We have recently identified interactions between two groups of Drosophila IgSF (immunoglobulin superfamily) cell adhesion molecules with properties closely matching a neuronal chemoaffinity function: 21 Dpr proteins, named after the founding member Defective proboscis extension response, selectively bind nine proteins, now called the Dpr-interacting proteins, or DIPs. All 21 Dprs and nine DIPs are predicted to contain two and three immunoglobulin (IG) domains, respectively. Our previous work identified the first IG domains, termed IG1, as the domains mediating the Dpr–DIP interaction by the formation of a pseudo-symmetric IG1-IG1 heterocomplex using the GFCC’C’ face of the immunoglobulin fold. Therefore, Dprs and DIPs are strong candidates for a synapse specification or targeting function.

We determined the crystal structure of Dpr10 IG1 bound to DIP-α IG1 and compared it to our Dpr6–DIP-α structure. The IG1 of Dpr6 and Dpr10 are 75% identical in sequence, and the interface only has three residues out of 19 that are different between Dpr6 and Dpr10. The two complex structures closely match each other, and unlike the differences among complexes described above, rotamers are nearly all conserved at the two interfaces. The differences in sequence are accommodated by small movements in surrounding side chains and do not propagate further. Overall, these results suggest that Dprs that are highly similar in sequence (≥70% identity) are unlikely to be differentiated in their DIP binding, but in time and place of expression. The high-resolution Dpr10–DIP-α structure also allowed us to observe an ordered, near-complete N-linked glycan at the interface. As we use lepidopteran cells to express Dprs and DIPs, the glycan structure and composition in our structure likely match the native insect Dpr/DIP glycans. The structure shows that the first N-acetyl glucosamine (NAG) is fucosylated at both the third and sixth carbon positions – commonly observed in arthropods but not in mammals. The glycan linked to Asn82 in Dpr10, which is present in seven out of 21 Dprs, is ordered as it inserts itself into a groove on the DIP-α surface, and adds a further 440 Å2 area to the buried surface area (total area: 2,240 Å2). Among the mutants tested in the mutational analysis of the Dpr10–DIP-α interface, the Dpr10 mutant Y103A abolishes DIP-α binding (orange box), and therefore can be used to study the Dpr10–DIP-α complex function, without effecting DIP-α homodimerization.

>GSWNEPYFDLTMPRNITSLVGKSAYLGCRVKHLGNKTVAWIRHRDLHILTVGTYTYTTDQRFQTSYHRDIDEWTLQIKWAQQRDAGVYECQISTQPVRSYSVNLNIVHHHHHH[2x];>[2x]SRAFQPEFVESISNVSVAVGRDATFTCHVRHLGGYRVGWLKADTKAIQAIHENVITHNPRVTVSHLDQNTWNLHIKAVSEEDRGGYMCQLNTDPMKSQIGFLDVVIPHHHHHH>ATPLTSLGSEQAMFHGKHQPGITTPMQARGHLVAFDLAAGAGRKEAAALLRRWSDTARRLMAGEPAGSRDTDVARDAGPSSLTVTFGFG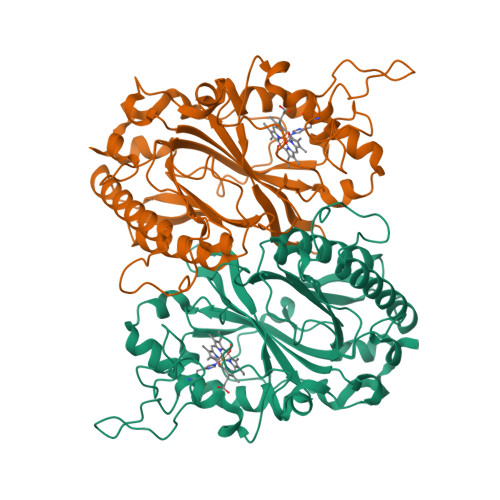HSFFGRTGLEKQRPVALDPLPDFSSDHLDKNRSNGDLWVQIGADDALVAFHALRAIQRDAGAAARVRWQMNGFNRSPGATAHPMTARNLMGQVDGTRNPKPGEADFDRRIFVPEEPEAGKGGPAWMANGSYVVVRRIRMLLDDWEELSLKAQEDVIGRRKSDGAPLSGGSGATESTEMDLEKTDGSGELVVPINAHARITRPDQNGGAAMVRRPFSYHDGFDADGVPDAGLLFVCWQADPLRGFVPVQRKLDRGDALSQFIRHEASGLFAVPGGAAEGEYVGQRLLE[2x]>MRLSYEALEWRTPIENSTEPVSLPPPPPFFGQERAREALELAIRGGFHAYLVGPPSLGKHEALLAYLSTQSV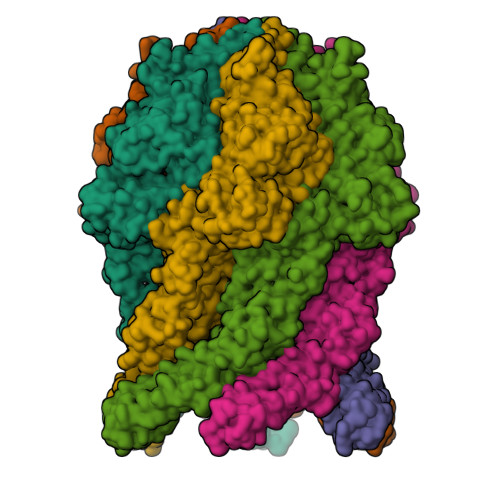ETPPDLLYVPLSERKVAVLTLPSGQEIHLAEAVEGLLLEVNRLDELFRQGSFLREKTQLEARFKEAREQQLEALRREAQEAGFALSTNGERLELTGPGPVPAELSARLEEVTLGSLAASAELEVALRRLRRDWALHYLNNRFEPLFQRFPQARAYLEALRARLARYAETGEPLDPAQWRPNLLTSSSSGTPPPIVYEPYATAPRLFGRLDYLVDRGVWSTNVSLIRPGAVHRAQGGYLILDALSLKREGTWEAFKRALRNGQVEPVTEPQAPAGLEVEPFPIQMQVILVGTPEAFEGLEEDPAFSELFRIRAEFSPTLPASPENCTALGGWLLAQGFQLTQGGLTRLYDEARRMAEQRDRMDARLVEIRALAEEAAVLGGGLLTAESVEQAIAAREHRSFLSEEEFLRAVQEGVIRLRTTGRAVGEVNSLVVVEAAPYWGRPARLTARAAPGRDHLISIDREAGLGGQIFHKAVLTLAGYLRSRYIEHGSLPVTISLAFEQNYVSIEGDSAGLAELVAALSAIGNLPLRQDLAVTGAVDQTGKVLAVGAINAKVEGFFRVCKALGLSGTQGVILPEANLANLTLRAEVLEAVRAGQFHIYAVETAEQALEILAGARMEGFRGLQEKIRAGLEAFARLEEGHDKEDREKLAAALEHHHHHH[6x]>[2x]GSEFRLEAERMRLAEEEKLRKEMSAKKA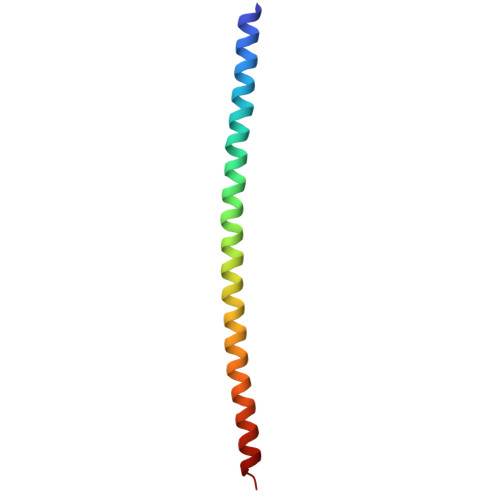KEEAERKHQERLAQLAREDAERELKEKEEARRKKELLEQMEKA cyclopentylacetic acid 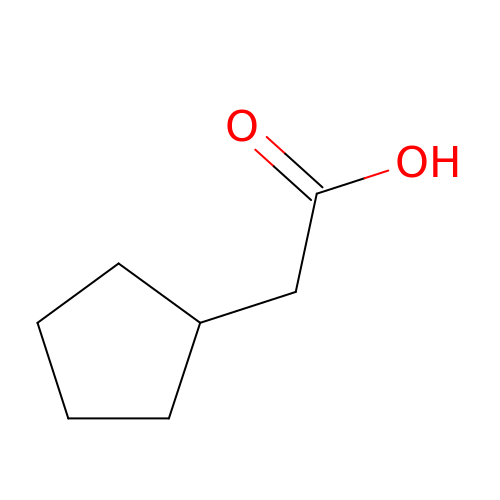| C7 H12 O2 | YVHAIVPPUIZFBA-UHFFFAOYSA-N4-naphthalen-1-yl-~{N}-oxidanyl-benzamide 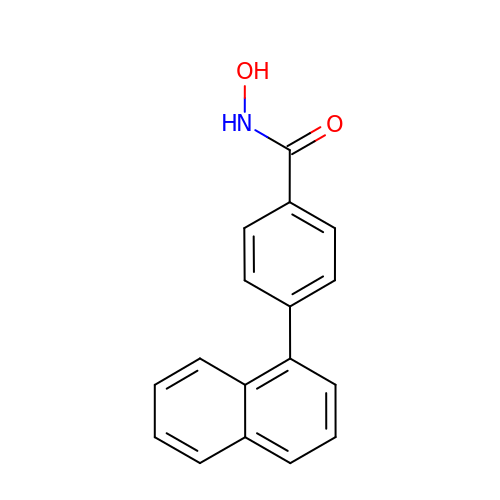| C17 H13 N O2 | PKQVYJOPUCLLCD-UHFFFAOYSA-N>[2x]MNINEILKKLINKSDLEINEAEELA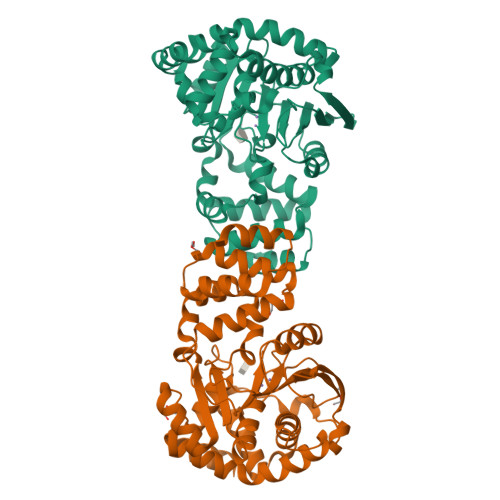KAIIRGEVPEILVSAILVALRMKGESKNEIVGFARAMRELAIKIDVPNAIDTAGTGGGGLGTVNVSTASAILLSLVNPVAKHGNRAVSGKSGSADVLEALGYNIIVPPERAKELVNKTNFVFLSAQYYHPAMKNVANVRKTLGIRTIFNILGPLTNPANAKYQLMGVFSKDHLDLLSKSAYELDFNKIILVYGEPGIDEVSPIGNTFMKIVSKRGIEEVKLNVTDFGISPIPIEKLIVNSAEDSAIKIVRAFLGKDEHVAEFIKINTAVALFALDRVGDFREGYEYADHLIEKSLDKLNEIISMNGDVTKLKTIVVKSSG>GMGSMAEKWEELSGKNNWEGLLNPLDLDLRKYIIQYGELAQATYDTFISERASKYAGASRYSMENFFTKVGLDPSKYHVTKFFYGTSSIPLPDAFMTRSLSREAWSKESNFMGWIAVATDEGKVALGRRDIVINWRGTLQVLEWVNDLQFLLVPAPKVFGDGGLLPLFHPLVHHGFHNIYTTENPRSQFNKTCVRDQVMEEVKRLVEEYKNEEVSITVTGHSLGASLATLNAVDIAFNGINKSSNGKEFPVTAFVFASPKVGDLNFHKAFSKLKHLHILRIHNLLDIVPKYPPVGYFDVGQELMIDTTKSPYVKPPGEVVSWHLLEPYLHGIAGTQGIGMTAGFKLEVNRDISLVNKQWMILKDEYCIPPLWWSEKHKGMVQQQDGSWLLQDRDDYEF[4x]

The phospholipases are classified into four groups according to the cleavage site; phospholipase A1 (PLA1) cleaves sn-1 acyl chain, phospholipase A2 (PLA2) cleaves sn-2 acyl chain, phospholipase C (PLC) cleaves before the phosphate, and phospholipase D (PLD) cleaves after the phosphate. Here, we report the first molecular structures of plant PLA1s: AtDSEL and CaPLA1 derived from Arabidopsis thaliana and Capsicum annuum, respectively. AtDSEL and CaPLA1 are divided into the following two domains: the α/β hydrolase domain containing the lid domain, GXSXG motif, and catalytic triad and the C-terminal domain containing the dimerization domain. In addition to the conserved α/β hydrolase scaffold, GXSXG motif, and catalytic triad, plant PLA1s have an extended C-terminal domain composed of approximately 70 residues.

CaPLA1 was selectively expressed in young roots of the hot pepper and hydrolyzed phospholipids at the sn-1 position. In the case of CaPLA1, there are four molecules in the asymmetric unit. Among the four molecules, two molecules make a homodimer; the other two molecules make homodimers with another symmetry mate, respectively. Each monomer of CaPLA1 has an overall structure similar to that of AtDSEL; α/β hydrolase domain and C-terminal domain are almost the same as each other. CaPLA1 also has two disconnected loops resulting from the disordered residues; Pro91 and Asp92 between β1 and β2 and from Asp160 to Phe167 between α6 and α7 could not be refined because of the deficient electron density map of the residues. The disordered residues from Asp160 to Phe167 affected the surrounding secondary structures; a pair of β-strands (β4 and β5 in the case of AtDSEL) were not found in CaPLA1. The AUC result of CaPLA1 also suggests that CaPLA1 makes homodimers in solution, considering that the molecular weight of the theoretical dimeric CaPLA1 and calculated from the AUC peak are 90.4 kDa and 86.0 kDa, respectively. The dimerization domain of CaPLA1 is similar to that of AtDSEL; however, more residues are involved in the dimerization. In CaPLA1, His376, Met379, and Trp387 of one monomer and Trp371 and Trp372 of the other monomer make hydrophobic interactions. Therefore, the dimeric interface of CaPLA1 is more robust than that of AtDSEL.>MERPQPDSMPQDLSEALKEATKEVHTQAENAEFMRNFQKGQVTRDGFKLVMASLYHIYVALEEEIERNKESPVFAPVYFPEELHRKAALEQDLAFWYGPRWQEVIPYTPAMQRYVKRLHEVGRTEPELLVAHAYTRYLGDLSGGQVLKKIAQKALDLPSSGEGLAFFTFPNIASATKFKQLYESRMNSLEMTPAVRQRVIEE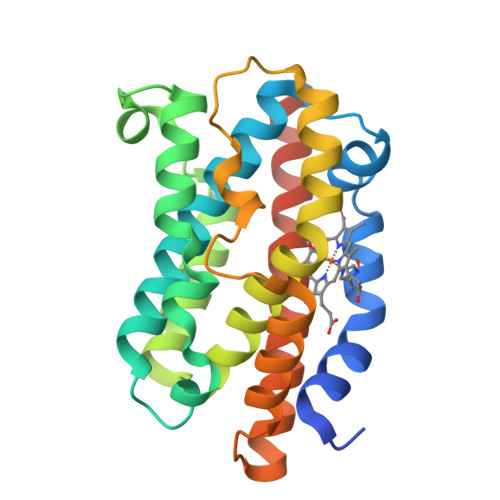AKTAFLLNIQLFEELQELLTHDTKDQSPSRA[2x]> MLDAFSKVITSADGKAAYVGGADLQALKKFVSDGNKRMDAVNAIVSNASCIVSDAVSGMVCENPSLIAPNGGVYSNRKMAACLRDAEIILRYVSYSLLSGDSSVLEDRCLNGLKETYSSLGVPAAGNARAVAIMKATVNSFINNTAQQKKLSVPS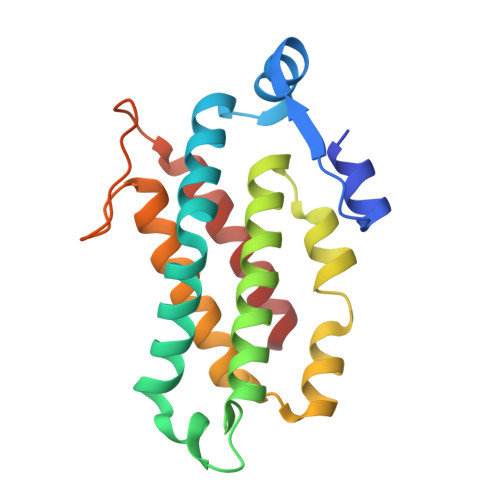GDCSALASEAGGYFDKVTSAIG>TRDA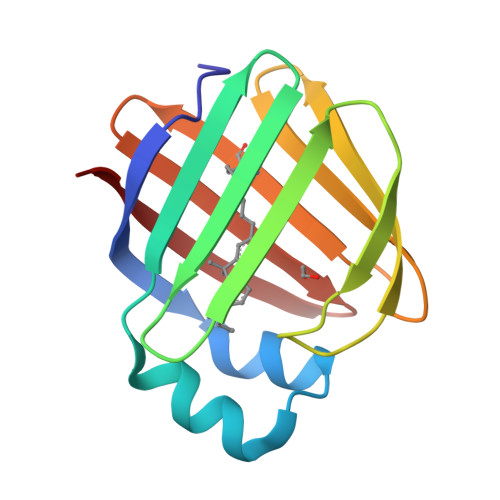NGTWEMESNENFEGWMKALDIDFALRKIAVRLTLTLVIDQDGDNFKVKCTSTFANYDVDFTVGVEFDEYTKSLDNRHVKALVTWEGDVLVCVQKGEKENRGWKKWIEGDKLYLELTCGDQVCRQVFKKK[2x]> SRNIHLLGRKTCLGRRVVQPGMFEDHPPTKKARVSMRR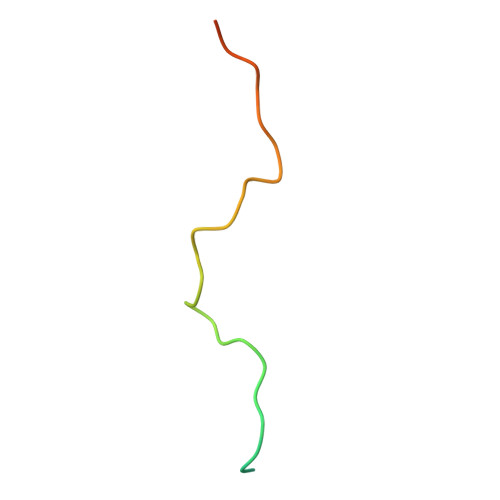MSN>SMVTIKVFSPKYPTELEEFYAERIADNPLGFIQRLDLLPSISGFVQKLREHGGEFFEMREGNKLIGICGLNPINQTEAELCKFHINSAYQSQGLGQKLYESVEKYAFIKGYTKISLHVSKSQIKACNLYQKLGFVHIKEEDCVVELGEETLIFPTLFMEKILS[3x]

HP0935 is a small (161 amino acids long) single GNAT domain-containing protein belonging to type IV protein acetyltransferases. A biochemical study showed that HP0935, the only known protein acetyltransferase in H. pylori, can acetylate free lysine amino acid and lysine residues in proteins. The crystal structure of HP0935 revealed a conserved GNAT fold, characteristic of the GNAT superfamily. The structure of HP0935 is composed of seven β-strands and four α-helices arranged in a topology—β1· α1· α2· β2· β3· β4· α3· β5· α4· β6· β7.

To gain structural insights, the crystal structures of HP0935 in its apo and ACO-bound forms were determined to be 2.00 Å and 2.40 Å resolution, respectively (see Experimental procedures). The apo- and ACO-bound HP0935 crystallized in distinct space groups, C2 and P61, respectively. A key observation was the partial disorder in the α1-α2 and complete disorder in the β6-β7 loop region in the apo-HP0935 structure, as evident from missing electron density. In apo-HP0935, the α1-α2 loop adopts an extended, distal conformation, positioned away from the ACO-binding cleft. In the distal conformation, two to three residues at the C-terminus of the loop are disordered, probably, due to the lack of stabilizing contacts. In apo-HP0935, this region remains disordered, exposed to solvent channels, whereas in ACO-HP0935, it is ordered as a β-hairpin and forms part of a β-sheet alongside β1, β2, and β3 from a symmetry-related molecule. Structural analysis of HP0935 identified E77 and H115 as potential general base residues and Y127 as a general acid. A conserved water molecule, hydrogen-bonded to L78, H115, and E77, was observed.Purine nucleoside phosphorylases (PNPs, EC 2.4.2.1) are cytosolic enzymes involved in the purine salvage pathway metabolism in most organisms. The enzyme degrades (2′-deoxy)nucleosides based on 6-oxopurines to the corresponding purine bases and (2-deoxy)ribose-1-phosphate. Purine nucleoside phosphorylase (PNP) is a well-known molecular target with potential therapeutic applications in the treatment of T-cell malignancies and/or bacterial/parasitic infections. The results are supported by a crystallographic study of eight enzyme-inhibitor complexes and by ADMET profiling in vitro and in vivo.

To obtain information on the binding pose and interacting residues, crystal structures of recombinant hPNP in complex with inhibitors 18c, 45b, 45q, 45i, and 45n were determined and refined to high resolution. All five inhibitors bind to hPNP in a similar way, i.e., through seven direct hydrogen bonds and four water-mediated hydrogen bonds as well as numerous hydrophobic interactions. Purine moiety forms three direct hydrogen bonds with the Glu201 sidechain, two bonds with sidechain Asn243, and two-waters-mediated hydrogen bonds with the main chain of Ile246. Central phenyl moiety is located in the pocket formed by Phe200, His257, and Phe159 provided by the neighboring molecule within the trimer. The phosphonate moiety of the inhibitor forms direct hydrogen bonds with side chains of Ser33 (except in 18c), Arg84, His86, and three water-mediated hydrogen bonds with Ala116, Tyr192, and Met219. Overall, the binding pose of inhibitors is comparable to immucilin H (ImmH),51 a PNP inhibitor currently approved in some countries for the treatment of peripheral T-cell lymphoma. Phosphonate moiety of compounds mimics the position of the phosphate ion in ImmH cocrystal structures and the position of the purine moiety is also conserved. To decipher structural reasons for different affinities of individual inhibitors, structure hPNP in complex with 18c can be used as a control to which the other four inhibitors are compared. The estimated Ki values for the selected hPNP inhibitor of the series, compound 18c, and for the reference inhibitor (forodesine) were 12 and 33 nM, respectively. For hPNP/18c, the reservoir contained 0.3 M magnesium chloride, 0.3 M calcium chloride, 20% w/v PEG 8000, 40% v/v ethylene glycol, 0.1 M MES/imidazole, and pH 6.0,53 and the drop consisted of 200 nL of protein, 80 nL of the precipitant solution, and 20 nL of 1 M ammonium sulfate (added as an additive).

>[6x]MENGYTYEDYKNTAEWLLSHTKHRPQVAIICGSGLGGLTDKLTQAQIFDYGEIPNFPRSTVPGHAGRLVFGFLNGRACVMMQGRFHMYEGYPLWKVTFPVRVFHLLGVDTLVVTNAAGGLNPKFEVGDIMLIRDHINLPGFSGQNPLRGPNDERFGDRFPAMSDAYDRTMRQRALSTWKQMGEQRELQEGTYVMVAGPSFETVAECRVLQKLGADAVGMSTVPEVIVARHCGLRVFGFSLITNKVIMDYESLEKANHEEVLAAGKQAAQKLEQFVSILMASIPLPDKAS> SPSSSEGGAFTVNMPKTSTVDDIRGCPTLETPLKLTFTEDIQPRKENGSTYFYYDGWRGVGQTVNPWSPVLDNHKYAATEHEIHIYVEFFQTPSNRFADKNGAYSYIDANGVMYTNGEYSWEHVPALGKNIYKVVISDWNKGQTKSIYLPGRDFKTVEVFHFQNNRPQWDDRNSYENVKSRINNNISKSYSKAKLNEQLSTYVHDDGTDSLFLYQKLSRASLKESQINYYQLRGKFNGVNLGYWAQEYILFGGEGAEQLKNKIPDMSNYSMEDNGSFKNALKIESLDLRLMDNNR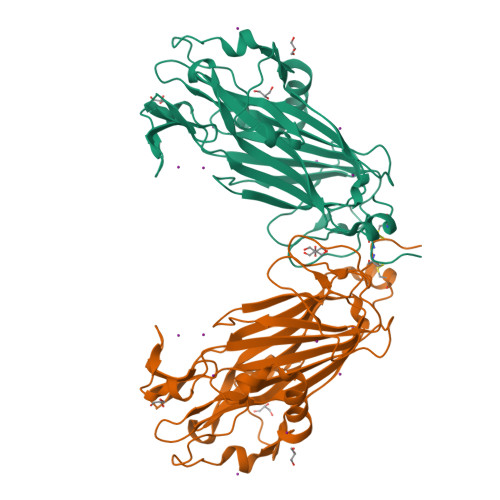MAYGSTGTYIASFNRTDFSMTPENLKACGLD> GMSQDNYFSRMLRGEAPVPAVAGTLGGVIR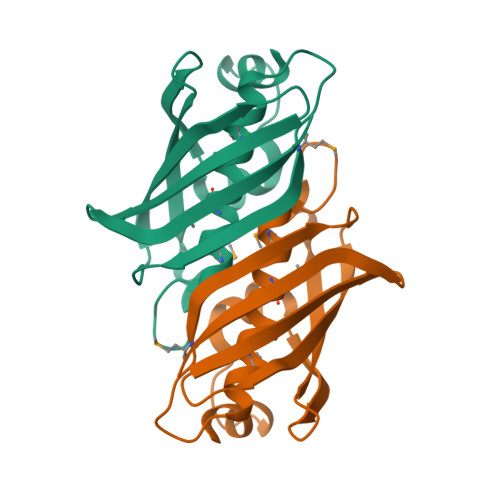AVDLEAGSLESDYVATDAFLNPVGQVQGGMLGAMLDDVTAMLVTATLEDGASCSTLNLNLSFLRPAQAGLLRGRARLERRGRNVCNVVGELSQDGKLVATATATCMVARRA>GMTYKDYTGLDRTELLSKVRHMMSDKRFNHVLGVERAAIELAERYGYDKEKAGLAALLHDYAKELSDDEFLRLIDKYQPDPDLKKWGNNIWHGLVGIYKIQEDLAIKDQDILAAIAKHTVGSAQMSTLDKIVYVADYIEHNRDFPGVEEAR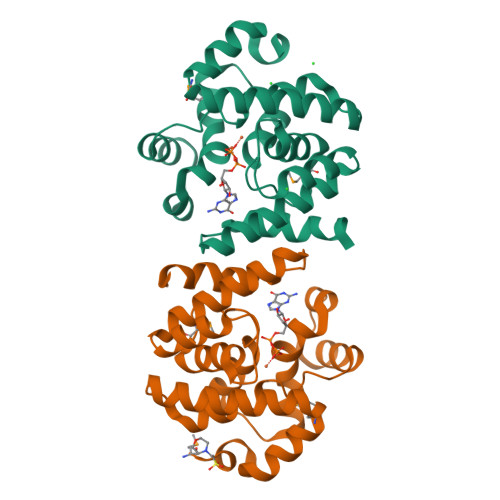ELAKVDLNKAVAYETARTVAFLASKAQPIYPKTIETYNAYIPYLD[2x]> DSGVDSGRPIGVVPFQWAGPGAA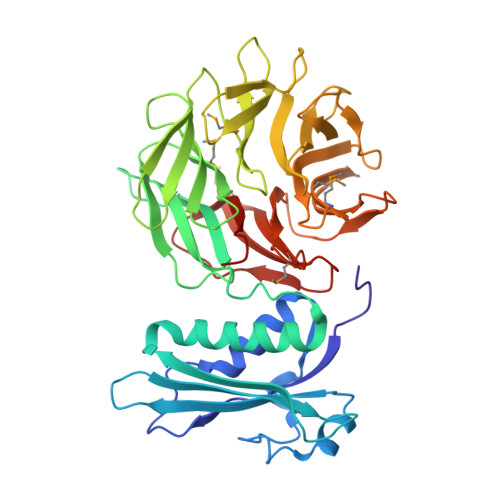PEDIGGIVAADLRNSGKFNPLDRARLPQQPGSAQEVQPAAWSALGIDAVVVGQVTPNPDGSYNVAYQLVDTGGAPGTVLAQNSYKVNKQWLRYAGHTASDEVFEKLTGIKGAFRTRIAYVVQTNGGQFPYELRVSDYDGYNQFVVHRSPQPLMSPAWSPDGSKLAYVTFESGRSALVIQTLANGAVRQVASFPRHNGAPAFSPDGSKLAFALSKTGSLNLYVMDLASGQIRQVTDGRSNNTEPTWFPDSQNLAFTSDQAGRPQVYKVNINGGAPQRITWEGSQNQDADVSSDGKFMVMVSSNGGQQHIAKQDLATGGVQVLSSTFLDETPSLAPNGTMVIYSSSQGMGSVLNLVSTDGRFKARLPATDGQVKFPAWSPYL>MDVSYLLDSLNDKQREAVAAPRSNLLVLAGAGSGKTRVLVHRIAWLMSVENCSPYSIMAVTFTNKAAAEMRHRIGQLMGTSQGGMWVGTFHGLAHRLLRAHHMDANLPQDFQILDSEDQLRLLKRLIKAMNLDEKQWPPRQAMWYINSQKDEGLRPHHIQSYGNPVEQTWQKVYQAYQEACDRAGLVDFAELLLRAHELWLNKPHILQHYRERFTNILVDEFQDTNNIQYAWIRLLAGDTGKVMIVGDDDQSIYGWRGAQVENIQRFLNDFPGAETIRLEQNYRSTSNILSAANALIENNNGRLGKKLWTDGADGEPISLYCAFNELDEARFVVNRIKTWQDNGGALAECAILYRSNAQSRVLEEALLQASMPYRIYGGMRFFERQEIKDALSYLRLIVNRNDDAAFERVVNTPTRGIGDRTLDVVRQTSRDRQLTLWQACRELLQE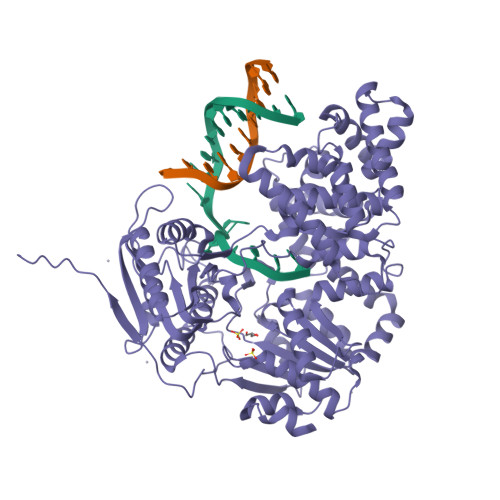KALAGRAASALQRFMELIDALAQETADMPLHVQTDRVIKDSGLRTMYEQEKGEKGQTRIENLEELVTATRQFSYNEEDEDLMPLQAFLSHAALEAGEGQADTWQDAVQLMTLHSAKGLEFPQVFIVGMEEGMFPSQMSLDEGGRLEEERRLAYVGVTRAMQKLTLTYAETRRLYGKEVYHRPSRFIGELPEECVEEVRLRATVSRPVSHQRMGTPMVENDSGYKLGQRVRHAK[2x]> MSNFKVRDPVIQERL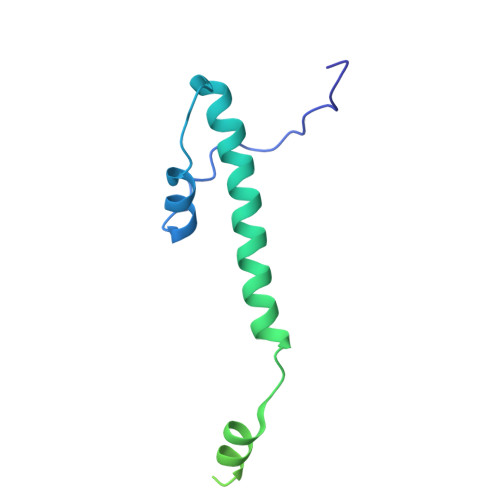DHDYAHHPLVARMNTLDQGNMSQAEYLVQKRHYLVFLIAHHYYEAYLRRMGGIQRRDHLQTLRDQKPRERADRVSAASAYDAGTFTVPSRPGPASGTTPGGQDSLGVSGSSITTLSSGPHSLSPASDILTTLSSTTETAAPAVADARKPPSGKKK> MDTNQKLSIAVFALGCFWGPDAQFGSIKGVVSTRVGYAGGTTNNPSYYNLGDHSESIEIQYDANVITYGELLNIFWNLHNPVYETTNRQYMSRIFYLDDGQKSEALEMKRQIEAANGEKIYTEIVPLENFYLAEGYHQKYYLQNTTKLYQT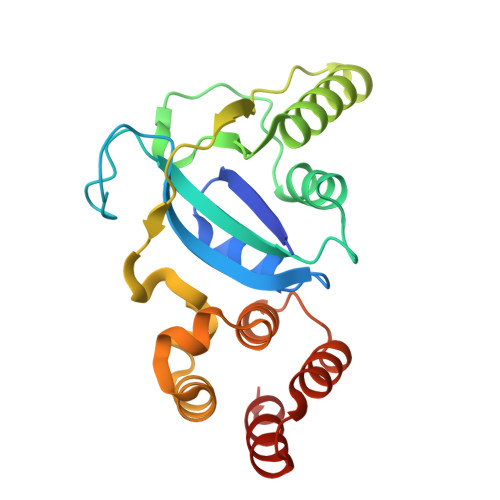LKAIYGGFGNLVRSTLAARMNGYIAGNLSIASLKEEMDLVELPEDQYEKVLSIVEEI> NTSDMYPMPNTLEYGNRTYKIINANMTWYAAIKTCLMHKAQLVSITDQYHQSFLTVVLNRLGYAHWIGLFT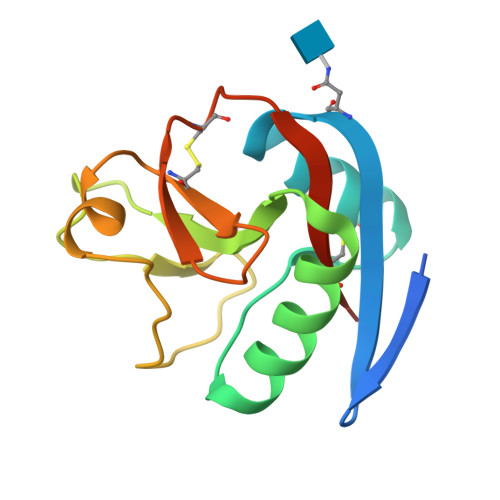TDNGLNFDWSDGTKSSFTFWKDEESSLLGDCVFADSNGRWHSTACESFLQGAICHVHHHHHH> MKTIIINGVQFNTDEDTTILKFARDNNIDISALCFLNNCNNDINKCEICTVEVEGTGLVTACDTLIEDGMIINTNSDAVNEKIKSRISQLLDIHEFKCGPCNRRENCEFLKLVIKYKARASKPFLPKDKTEYVDERSKSLTVDRTKCLLCGRCVNACGKNTETYAMKFLNKNGKTIIGAEDEKCFDDTNCLLCGQCIIACPVAALSEKSHMDRVKNALNAPEKHVIVAMAPSVRASIGELFNMGFGVDVTGKIYTALRQLGFDKIFDINFGADMTIMEEATELVQR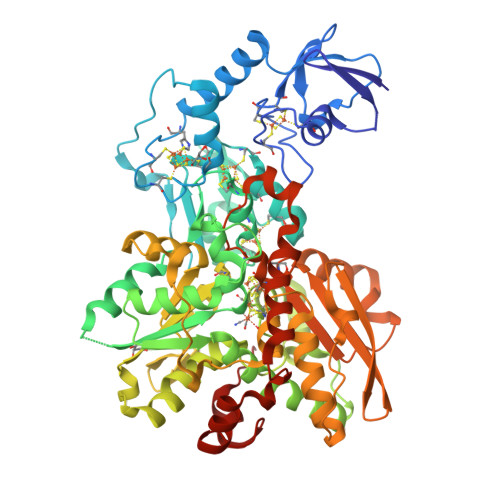IENNGPFPMFTSCCPGWVRQAENYYPELLNNLSSAKSPQQIFGTASKTYYPSISGLDPKNVFTVTVMPCTSKKFEADRPQMEKDGLRDIDAVITTRELAKMIKDAKIPFAKLEDSEADPAMGEYSGAGAIFGATGGVMEAALRSAKDFAENAELEDIEYKQVRGLNGIKEAEVEINNNKYNVAVINGASNLFKFMKSGMINEKQYHFIEVMACHGGCVNGGGQPHVNPKDLEKVDIKKVRASVLYNQDEHLSKRKSHENTALVKMYQNYFGKPGEGRAHEILHFKYKK> GHMGSSGGKQVERMPSE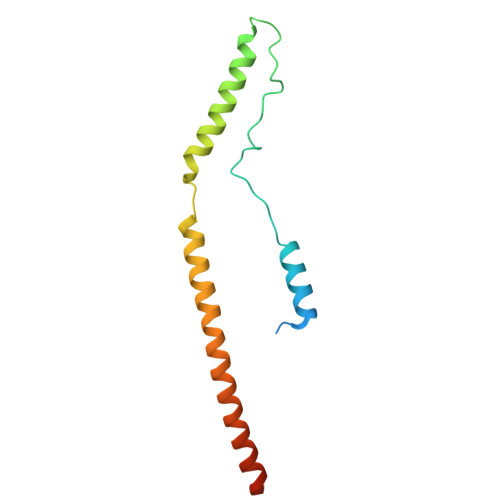RIPHSFFTQWNSELDGSVRMEDDGSREIPCPPTFCLTDCNDKDTVDSMYKYARKLSSLQNSSEEGPSSTLLTMIRQYMMEADYQRVEIARLKDSLNDKDEEIKKLRGFCSRYKRENA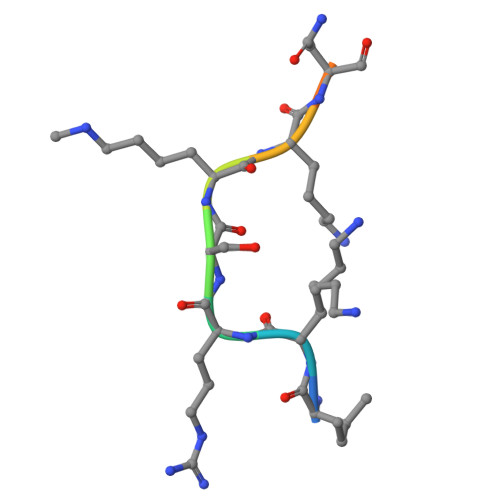> IKRSKKNSLA>[2x]GSHMPIEDV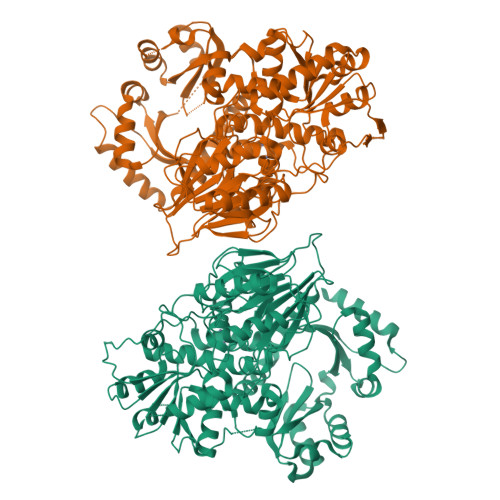LLDLKHKIEKNLPAGVTITDVEFEGPQLVLYTEEPRKFADDGNIIRNLAKELRTRIAMRPDPRVLATPEDSISIIEEVVPKESVISSYYFDPDSGEVIIEAEKPGLVIGKHGATLREITKQIGWIPKVVRTPPIKSRTVKNIREFMRNNLKERKEILKTVGRKIHRECTSKDQWVRVTALGGCKEVGRSCFLLSTPESRILIDCGVNVGSDENMTPYLYVPEVFPLNQIDAVIVTHAHLDHQGLVPLLFKYGYEGPVYCTPPTRDLMVLLQLDYIDVAAKEGKKIPYESGMVAKTLKHTIPLDYEEVTDIAPDIKLTFHNAGHILGSAISHFHIGDGLHNVVFTGDYKYEKTRLFDPAVNKFPRVETVISEATYGNANAFQPALKDAEKHLQMVVKNTIERGGIAVIPAFAVGRSQEVMIVLEESIRKGLIPEVPVYLDGMIWEATAIHATHPEYLNNDLRKLIFQKGQNPFLSECFKPVDSHEARQKIIQNPQPCVILATSGMMNGGPVMEYFKAFAEDPRNTLVFVGYQADGTIGRRIQKGWKEIPMTGKNGSTEMLKMNMEVQVVDGFSGHSDRRQLMEYVKRMQPRPERVFTEHGDEKACVDLASSVYKKLKIETRALTNLETVRLL> LEVLFQGPLGSPEFPGRLERPHMTAIAPVITVDGPSGAGKGTLCKALAESLNWRLLDSGAIYRVLALAALHHQVDISTEEALVPLAAHLDVRFVSQNGQLQVILEGEDVSNEIRTETVGNTASQAAAFPRVREALLRRQRAFREAPGLIADGRDMGTIVFPDAPVKIFLDASSQERAHRRMLQLQERGFNVNFERLLAEIQERDNRD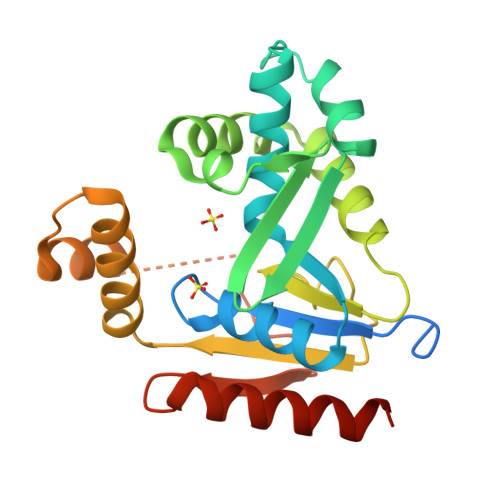RNRSVAPLVPAADALVLDSTSMSIEQVIEQALAYAQRILALPLKK> SEISRVYEAYPEKKATLYFLVLGFLALIVGSLFGPFQALNYGNVDAYPLLMHHHHHHAVRASEISRVYEAYPEKKATLYFLVLGFLALIVGSLFGPFQALNYGNVDAYPLLKRLLPFVQSYYQGLTLHGVLNAIVFTQLFAQAIMVYLPARELNMRPNMGLMWLSWWMAFIGLVVAALPLLANEATVLYTFYPPLKGHWAFYLGASVFVLSTWVSIYIVLDLWRRWKAANPGKVTPLVTYMAVVFWLMWFLASLGLVLEAVLFLLPWSFGLVEGVDPLVARTLFWWTGHPIVYFWLLPAYAIIYTILPKQAGGRLVSDPMARLAFLLFLLLSTPVGFHHQFADPGIDPTWKMIHSVLTLFVAVPSLMTAFTVAASLEFAGRLRGGRGLFGWIRALPWDNPAFVAPVLGLLGFIPGGAGGIVNASFTLDYVVHNTAWVPGHFHLQVASLVTLTAMGSLYWLLPNLTGKPISDAQRRLGLAVVWLWFLGMMIMAVGLHWAGLLNVPRRAYIAQVPDAYPHAAVPMVFNVLAGIVLLVALLLFIYGLFSVLLSRERKPELAEAPLPFAEVISGPEDRRLVLAMDRIGFWFAVAAILVVLAYGPTLVQLFGHLNPVPGWRLW;> DQHKAHKAILAYEKGWLAFSLAMLFVFIALIAYTLATHTAGVIPAGKLERVDPTTVRQEGPWADPAQAVVQTGPN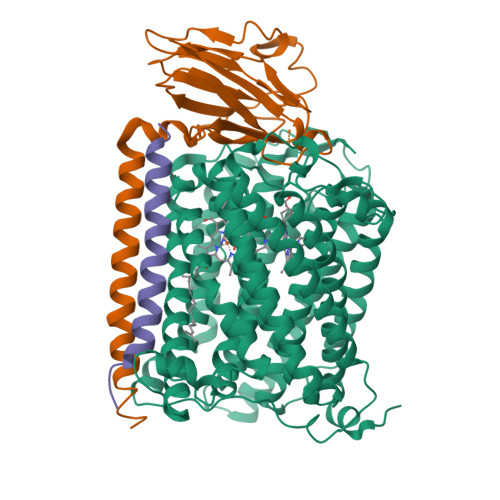QYTVYVLAFAFGYQPNPIEVPQGAEIVFKITSPDVIHGFHVEGTNINVEVLPGEVSTVRYTFKRPGEYRIICNQYCGLGHQNMFGTIVVKE;> EEKPKGALAVILVLTLTILVFWLGVYAVFFARG>APMGSDPPTACCFSYTARKLPRNFVVDYYETSSLCSQPAVVFQTKRS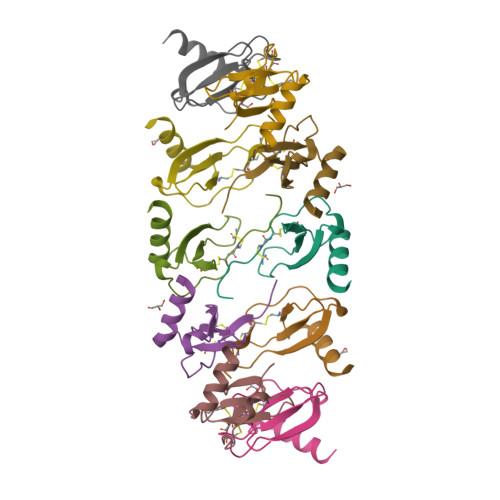KQVCADPSESWVQEYVYDLELN[5x]> GPGVCKSYKSVALVVGVTGIVGSSLAEVLKLPDTPGGPWKVYGVARRPCPVWLAKKPVEYIQCDVSNNQETISKLSPLKDITHIFYVSWIGSEDCQTNATMFKNILNSVIPNASNLQHVCLQTGIKHYFGIFEEGSKVVPHDSPFTEDLPRLNVPNFYHDLEDILYEETGKNNLTWSVHRPALVFGFSPCSMMNIVSTLCVYATICKHENKALVYPGSKNSW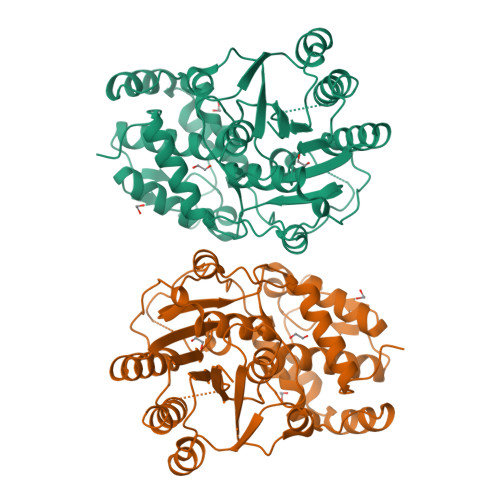NCYADAVDADLVAEHEIWAAVDPKAKNQVLNCNNGDVFKWKHIWKKLAEEFGIEMVGYVEGKEQVSLAELMKDKDQVWDEIVKKNNLVPTKLKEIAAFWFADIAFCSENLISSMNKSKELGFLGFRNSMKSFVSCIDKMRDYRFIPKAF Aberrant regulation of the PI3K/AKT pathway is implicated in the pathogenesis of several human cancers and inhibitors for multiple targets in this pathway are in clinical trials for the treatment of cancer. The PH domain directs AKT translocation from the cytosol to the plasma membrane by binding to the membrane lipids phosphatidylinositide (PtdIns)(3,4)P2 and PtdIns(3,4,5)P3, which are products of phosphatidylinositide-3-kinase (PI3K). AKT is subsequently phosphorylated resulting in kinase activation. Comprehensive and elegant experimentation revealed substantial differences in the relative positions of the PH and kinase domains of inactive and membrane-associated AKT, resulting in the inactive form being termed the closed or ‘PH-in’ conformation; whereas the membrane-associated form is referred to as the open or ‘PH-out’ conformation.

We were able to co-crystallize ΔHM-AKT1(1–443) with Inhibitor VIII and to solve its structure to 2.7 Å resolution. The PH domain nestles between the N- and C-lobes of the kinase domain with Inhibitor VIII binding to all three regions. The superimposed structures show the PH domain fills part of the space occupied by the αC-helix and phosphorylated activation loop in the activated AKT kinase domain structures; thereby sterically preventing the kinase domain from attaining an active conformation. Inhibitor VIII binds to AKT1 in an allosteric binding site formed at the combined interface of the PH domain and the N- and C- lobes of the kinase domain. We were pleased to observe a ring-stacking interaction between Inhibitor VIII and Trp 80 as an alanine mutation of this residue in AKT1 has been shown to render Inhibitor VIII inactive. Ser 205 has the only direct hydrogen bond to Inhibitor VIII. We did not observe Glu 17 binding to the inhibitor in the co-crystal structure, however Glu 17 forms a salt bridge with the positively charged kinase residue Arg 273 almost certainly providing additional stabilization to the closed ‘PH-in’ conformation. The conformation of the ATP binding site in the AKT1:Inhibitor VIII crystal structure clearly shows that the PH-in conformer is unable to bind ATP or ATP-competitive inhibitors. In contrast, the AKT1:Inhibitor VIII co-crystal structure reveals the allosteric inhibitor locking AKT into a closed conformation with its phospholipid binding site blocked by the kinase domain.

> GAMASDVAIVKEGWLHKRGEYIKTWRPRYFLLKNDGTFIGYKERPQDVDQREAPLNNFSVAQCQLMKTERPRPNTFIIRCLQWTTVIERTFHVETPEEREEWTTAIQTVADGLKKQEEEEMDFRSGSPSDNSGAEEMEVSLAKPKHRVTMNEFEYLKLLGKGTFGKVILVKEKATGRYYAMKILKKEVIVAKDEVAHTLTENRVLQNSRHPFLTALKYSFQTHDRLCFVMEYANGGELFFHLSRERVFSEDRARFYGAEIVSALDYLHSEKNVVYRDLKLENLMLDKDGHIKITDFGLCKEGIKDGATMKTFCGTPEYLAPEVLEDNDYGRAVDWWGLGVVMYEMMCGRLPFYNQDHEKLFELILMEEIRFPRTLGPEAKSLLSGLLKKDPKQRLGGGSEDAKEIMQHRFFAGIVWQHVYEKKLSPPFKPQVTSETDTRYFDEEFT>[4x]MTDTPFIRPDMKAFLEAIAAMAGPTLAEMTLEEARASYVALHGMADRPARELAVIRNLSCPGPAGDIPLRLYDARESREAGPVITFYHGGGFVIGDLDTHHNLCTEIAALMDLPVVAVDYRLAPEHPFPAAIEDC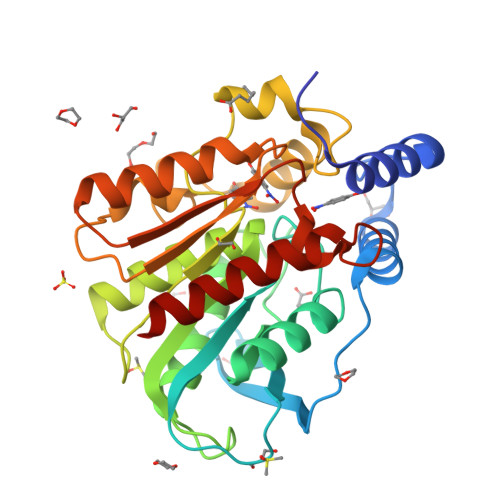EAATRWVASSPSELGRTASGVIPIGDAAGGNATIVVSQLLGAKPADVPVVLQVPIFPLASDAVGSASLEAFAEGFVLTKASIEFFDTAYKADRADPRGFPILGDHTAAPPTIVATASLDPIRDSGRDYAKALVEAGRDVVYLEMEGVTHSFTNIRAAVPSTQGDLERIIAAMKMMLGTA> A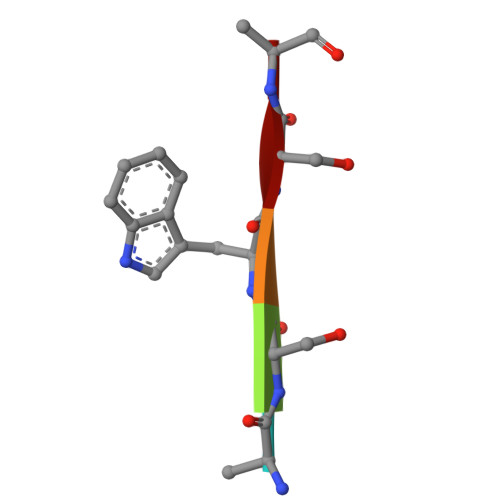SWSA> GSHMEAVQNRIVEAAERVPGVRGVIHLRARYVGQDIWAAMIIGVDPENTVEQAHEICEAVQAAVCGKIRRIESLAVSAEAREIGDTTKPSFSDQPLSFDEVMLSKVDN

One group of metal ion efflux transporters that regulates metal ion homeostasis and can be found in all domains of life is the Cation Diffusion Facilitator (CDF) protein family. One of the most highly conserved and abundant integral MM proteins is the CDF transporter MamM. MamM was recently proposed to function as a magnetosome-directed iron transporter required for iron biomineralization since its deletion abolished magnetite biomineralization and mutation of residues within the conserved TMD metal-binding site resulted in alterations of magnetite crystal size, morphology and even mineral phase. To summarize our results we present an alternative model for the CDF CTD mode of action, in which we propose that upon metal cation binding, the CTD induces conformational changes towards a tighter and more compact fold which allows the activation of iron transport through the TMD.

To gain a better understanding of the contribution of these binding sites to protein function two double alanine point mutations were also analyzed. In vivo the introduction of double point mutations in the central putative binding site (D249A and H285A) resulted in decreased Cmag values similar to D249A. Although the average particle number per cell was almost identical between the D249A and the D249A + H285A strains, the latter strain produced particles with significantly reduced mean diameters (−12%, P<0.001, Mann-Whitney test). In addition, this strain also showed a slower restoration of its magnetic response upon induction of biomineralization by adding iron back to iron-starved cells. ITC results for the central putative binding site double mutant (D249A and H285A) displayed a reduced number of binding sites (1.8±0.2) in reference to the wild-type data and therefore suggests that a single cation binds to each peripheral binding site. To confirm that these observed phenotypic differences are due to true transport function alternations, we also examined the expression levels of all MamM mutants, their ability to stabilize MamB expression, performed MD simulations for dimer stability evaluation and determined their CTD structures. (ii) All mutants exhibited an apo-MamM CTD-like behavior along the MD simulations (see Fig. B in file S1 for representative MD simulations), and (iii) an absence of structural differences was observed.> MSDMN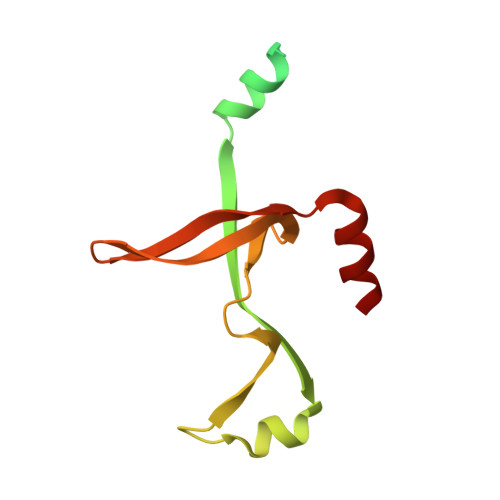NPSDENTGALDDLWADALNEQKATTTKSAADAVFQQLGGGDVSGAMQDIDLIMDIPVKLTVELGRTRMTIKELLRLTQGSVVALDGLAGEPLDILINGYLIAQGEVVVVADKYGVRITDIITPSERMRRLSR> CPSRCSCSGTEIRCNSKGLTSVPTGIPSSATRLELESNKLQSLPHGVFDKLTQLTKLSLSQNQIQSLPDGVFDKLTKLTILYLHENKLQSLPNGVFDKLTQLKELALDTNQLKSVPDGIFDRLTSLQKIWLHTNPWDCSCPR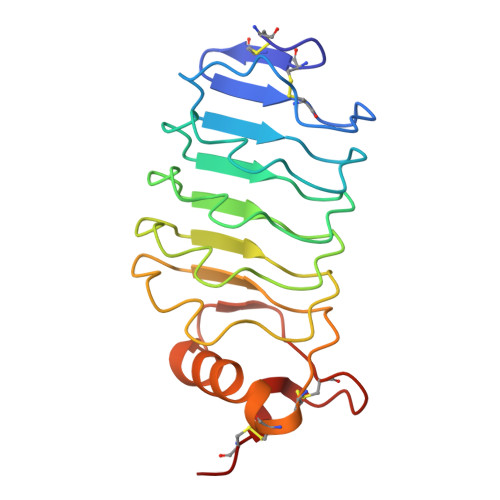IDYLSRWLNKNSQKEQGSAKCSGSGKPVRSIICPT>RSNLAIYWGQGPNQLRLSHFCQETSLDIINIGFINYFPDMSPGHWPGSNFGNQCDGSVYVTNDGVVTKLLSGCHQIMEDIPICQAAGKKVLLSIGGAYPPDQSILSEDSAVAFATFLWGAFGPVAEGWEGPRPFGDVVVDGFDFDIEHNGGFGYATMVNTFRQYFNQVPERKFYLSAAPQCIIPDAQLSDAIFNAAFDFIWIQYYNTAACSAKSF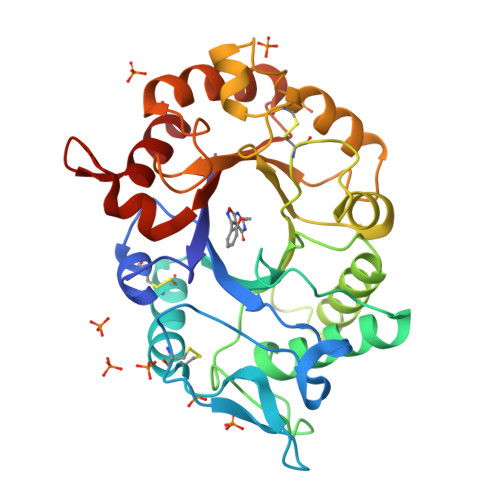IDTSLGTFNFDAWVTVLKASASKDAKLYVGLPASETAANQGYYLTPDEVESLVSTYMDRYPDTFGGIMLWEATASENNQIDGAPYADHMKDILLH[2x]> PQAKYRHDYRAPDYQITDIDLTFDLDAQKTVVTAVSQAVRHGASDAPLRLNGEDLKLVSVHINDEPWTAWKEEEGALVISNLPERFTLKIINEISPAANTALEGLYQSGDALCTQCEAEGFRHITYYLDRPDVLARFTTKIIADKIKYPFLLSNGNRVAQGELENGRHWVQWQDPFPKPCYLFALVAGDFDVLRDTFTTRSGREVALELYVDRGNLDRAPWAMTSLKNSMKWDEERFGLEYDLDIYMIVAVDFFNMGAMENKGLNIFNSKYVLARTDTATDKDYLDIERVIGHEYFHNWTGNRVTCRDWFQLSLKEGLTVFRDQEFSSDLGSRAVNRINNVRTMRGLQFAEDASPMAHPIRPDMVIEMNNFYTLTVYEKGAEVIRMIHTLLGEENFQKGMQLYFERHDGSAATCDDFVQAMEDASNVDLSHFRRWYSQSGT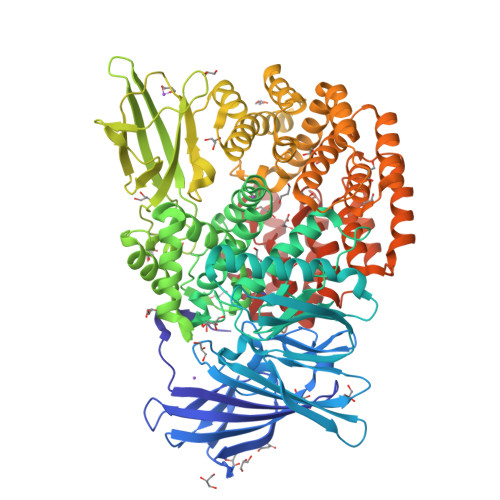PIVTVKDDYNPETEQYTLTISQRTPATPDQAEKQPLHIPFAIELYDNEGKVIPLQKGGHPVNSVLNVTQAEQTFVFDNVYFQPVPALLCEFSAPVKLEYKWSDQQLTFLMRHARNDFSRWDAAQSLLATYIKLNVARHQQGQPLSLPVHVADAFRAVLLDEKIDPALAAEILTLPSVNEMAELFDIIDPIAIAEVREALTRTLATELADELLAIYNANYQSEYRVEHEDIAKRTLRNACLRFLAFGETHLADVLVSKQFHEANNMTDALAALSAAVAAQLPCRDALMQEYDDKWHQNGLVMDKWFILQATSPAANVLETVRGLLQHRSFTMSNPNRIRSLIGAFAGSNPAAFHAEDGSGYLFLVEMLTDLNSRNPQVASRLIEPLIRLKRYDAKRQEKMRAALEQLKGLENLSGDLYEKITKALA>GTTGGGGTTGGGGTTGGGGTTGGGG[4x]

G-quadruplexes (GQs) are non-canonical DNA structures composed of stacks of stabilized G-tetrads. Telomeres are repetitive, G-rich DNA sequences that exist at the ends of linear chromosomes and aid in their stabilization and protection. In this work, we focus on the telomeric repeat from Tetrahymena thermophila (referred to as TET) which has the overall sequence (TTGGGG)n. Furthermore, we report four high-resolution K+-stabilized crystal structures of two variants, TET25 (one structure) and TET26 (three structures).

While TET25 in solution exists as a mixture of three conformations, only the major hybrid [3 + 1] conformation crystallized. The crystals belong to the P1211 space group and diffract to 1.56 Å resolution. The ASU contains four unambiguously positioned copies of four-tetrad hybrid GQs, two spermine molecules, three K+ per GQ (12 K+ in total), and six Mg2+ ions, Supplementary Figure S5A. According to the GQ topology classification by Webba de Silva, TET25’s conformation is most similar to type V-9b, a hybrid [3 + 1] GQ. G1, G4, G16-G18 and G22 adopt syn glycosidic conformations, while all other guanines adopt anti glycosidic conformations. The most interesting aspect of the structure is the involvement of the 5′-G1(syn) from the 5′-GTT overhang in the top G-tetrad formation along with G19(anti)–G22(syn)–G4(syn). G1 displaces G13, which is part of the second GGGG stretch, into the lateral GTT loop. Therefore, in addition to two lateral loops and one propeller loop typically seen in V-9b structures, TET25 exhibits another lateral loop (overall three lateral loops and one propeller loop). The unique structural feature of a non-G-stretch guanine participating in a tetrad formation is called a snapback, in this case a 5′-top snapback, Figure 3E. TET25 has three lateral loops (T2–T3, G13–T14–T15, and T20–T21) and one propeller loop (T8–T9). The central ion channel contains three K+ ions in a square antiprismatic coordination with eight O6 carbonyl oxygens of guanines.> YTPVEEKENGRMIVIVAKKYEGDIKDFVDWKNQRGLRTEVKVAEDIASPVTANAIQQFVKQEYEKEGNDLTYVLLVGDHKDIPAKITPGIKSDQVYGQIVGNDHYNEVFIGRFSCESKEDLKTQIDRTIHYERNITTEDKWLGQALCIASAEGGPSADNGESDIQHENVIANLLTQYGYTK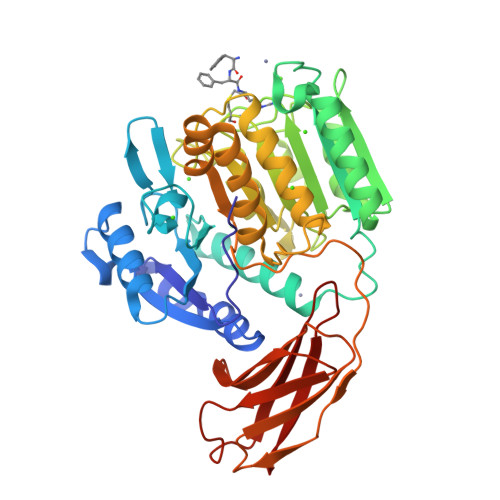IIKCYDPGVTPKNIIDAFNGGISLVNYTGHGSETAWGTSHFGTTHVKQLTNSNQLPFIFDVACVNGDFLFSMPCFAEALMRAQKDGKPTGTVAIIASTIDQYWAPPMRGQDEMNEILCEKHPNNIKRTFGGVTMNGMFAMVEKYKKDGENMLDTWTVFGDPSLLVRTLVPTEMQVTAPANISASAQTFEVACDYNGAIATLSDDGDMVGTAIVKDGKAIIKLNESIADETNLTLTVVGYNKVTVIKDVKVEGTS Prochloraz | C15 H16 Cl3 N3 O2 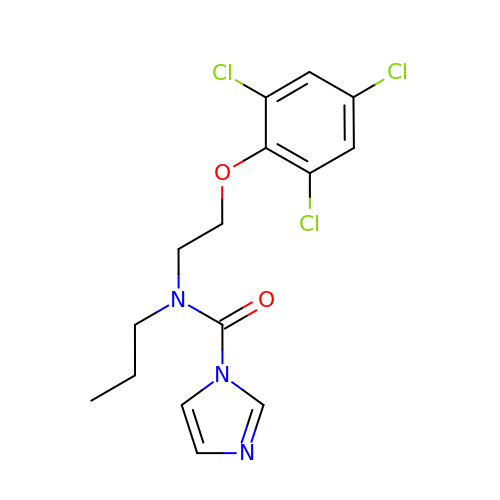| TVLSRXXIMLFWEO-UHFFFAOYSA-N>GQDRLDAPPPPAPPLLRWAGPVGVSWGLRAAAPGGPVPRAGRWRRGAPAEDQDCGRLPDFIAKLTNNTHQHVFDDLSGSVSLSWVGDSTGVILVLTTFQVPLVIVSFGQSKLYRSEDYGKNFKDITNLINNTFIRTEFGMAIGPENSGKVILTAEVSGGSRGGRVFRSSDFAKNFVQTDLPFHPLTQMMYSPQNSDYLLALSTENGLWVSKNFGEKWEEIHKAVCLAKWGPNNIIFFTTHVNGSCKADLGALELWRTSDLGKTFKTIGVKIYSFGLGGRFLFASVMADKDTTRRIHVSTDQGDTWSMAQLPSVGQEQFYSILAANEDMVFMHVDEPGDTGFGTIFTSDDRGIVYSKSLDRHLYTTTGGETDFTNVTSLRGVYITSTLSEDNSIQSMITFDQGGRWEHLRKPENSKCDATAKNKNECS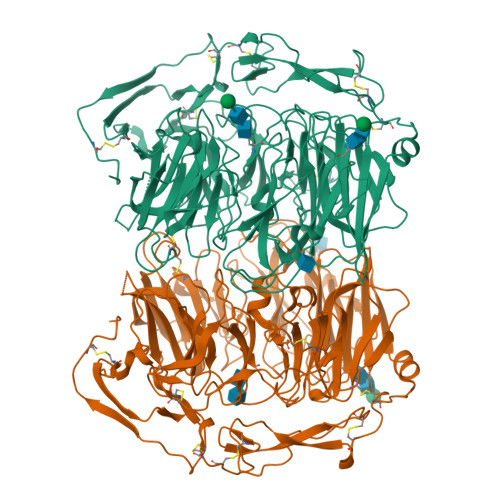LHIHASYSISQKLNVPMAPLSEPNAVGIVIAHGSVGDAISVMVPDVYISDDGGYSWAKMLEGPHYYTILDSGGIIVAIEHSNRPINVIKFSTDEGQCWQSYVFTQEPIYFTGLASEPGARSMNISIWGFTESFITRQWVSYTVDFKDILERNCEEDDYTTWLAHSTDPGDYKDGCILGYKEQFLRLRKSSVCQNGRDYVVAKQPSVCPCSLEDFLCDFGYFRPENASECVEQPELKGHELEFCLYGKEEHLTTNGYRKIPGDKCQGGMNPAREVKDLKKKCTSNFLNPTKQNSKSNAAAHHHHHH[2x]The TLP Gentlyase, the neutral metalloprotease from Paenibacillus polymyxa (EC 3.4.24.28), is an extracellular metalloprotease that cleaves fibronectin, collagen IV and, to a lesser extent, collagen and has maximum activity at neutral pH. This enzyme is used to gently disperse mammalian cells and tissues and is widely applied in cell-culture procedures or for the isolation and tissue dissociation of primary cells. The Gentlyase metalloprotease structure shows the overall architecture of a typical TLP. The C-terminal and N-terminal domains are connected by a central α-helix containing several catalytically crucial residues.

Here, we report (i) a method that can be generally applied to identify suitable conditions to keep active TLP stable for crystallization and (ii) the structure of Gentlyase, the TLP of P. polymyxa, at 1.59 Å resolution in the absence of and at 1.76 Å resolution in the presence of phosphoramidon, the natural TLP inhibitor from Streptomyces tanashiensis. Sadly, the pair of Gentlyase structures described here do not help in clarifying the question of whether the domain movement upon inhibitor binding is a general feature of all Bacillus TLPs. The lack of domain movement observed for the Gentlyase metalloprotease can be explained by the dipeptide fortuitously bound to the active site in the uninhibited form. The same rationale was applied to explain the lack of movement originally observed for thermolysin, in which the un­inhibited crystals also showed electron density for a dipeptide. In the uninhibited Gentlyase crystal the observed electron density for a dipeptide does not perfectly fit the side chains of any canonical amino acids. We used a Thr-Lys dipeptide model for refinement, which explains the electron density less poorly than Val-Lys. However, the observed electron density is likely to represent a mixture of proteolysis and autolysis products. The same Tyr150 position was observed as an alternative conformation in our structure of the uninhibited Gentlyase metalloprotease, indicating its possible physiological relevance. Another possible explanation for the lack of domain movement observed in the Gentlyase structure is the loss of the double glycine motif that precedes the central helix and is close to the thermolysin-like protease hinge-bending axis reported by Holland et al.. Comparison with other TLPs showed that the marked calcium dependency of Gentlyase stability may arise from a partly degenerated calcium site Ca1–2 and a deletion near site Ca3.

>[2x]ATGTGKGVLGDTKSFTTTASGSSYQLKDTTRGNGVVTYTASNRQSIPGTILTDADNVWNDPAGVDAHTYAAKTYDYYKAKFGRNSIDGRGLQLRSTVHYGSRYNNAFWNGSQMTYGDGDGSTFIAFSGDPDVVGHELTHGVTEYTSNLEYYGESGALNEAFSDVIGNDIQRKNWLVGDDIYTPNIAGDALRSMSNPTLYDQPDHYSNLYTGSSDNGGVHTNSGIINKAYYLLAQGGTFHGVTVNGIGRDAAVQIYYSAFTNYLTSSSDFSNARAAVIQAAKDQYGANSAEATAAAKSFDAVGVN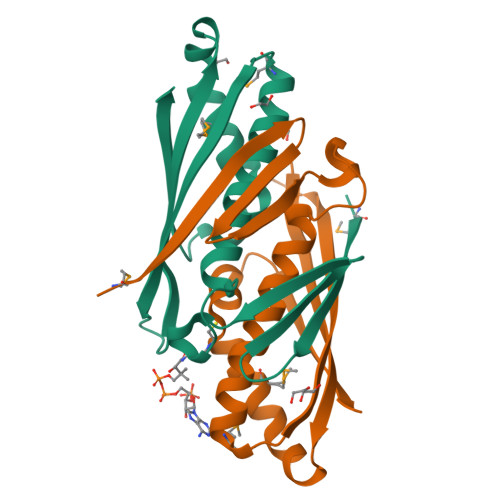>[2x]GMHVYESDVSWIDDRRTEVSVGDHRIEVDSPPEFGGPEGQLYPETLFPSVLASCLLTTFLEFKDRMGINLKSWNSHVTAELGPSPEKGFKFHRIKIHVKIGVNDEDKEKIPRAMQLAEKYCFISRAIRNNVEEIVDYEFV> TSWSDRLQNAADMPANMDKHALKKYRREAYHRVFVNRSLAMEKIKCFGFNMDYTLAVYKSPEYESLGFELTVERLVSIGYPQELLSFAYDSTFPTRGLVFDTLYGNLLKVDAYGNLLVCAHGFNFIRGPETREQYPNKFIQRDDTERFYILNTLFNLPETYLLACLVDFFTNCPRYTSCETGFKDGDLFMSYRSMFQDVRDAVDWVHYKGSLKE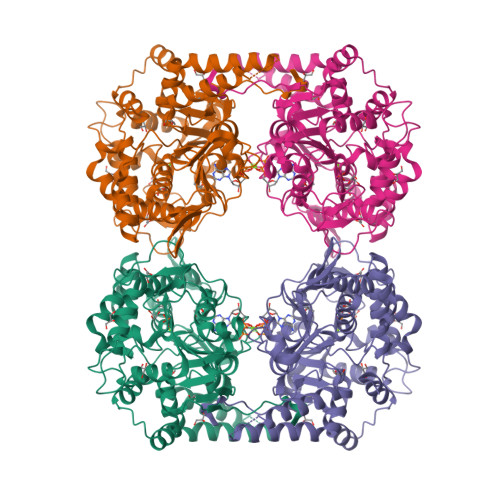KTVENLEKYVVKDGKLPLLLSRMKEVGKVFLATNSDYKYTDKIMTYLFDFPHGPKPGSSHRPWQSYFDLILVDARKPLFFGEGTVLRQVDTKTGKLKIGTYTGPLQHGIVYSGGSSDTICDLLGAKGKDILYIGDHIFGDILKSKKRQGWQTFLVIPELAQELHVWTDKSSLFEELQSLDIFLAELYKHLDSSSIQRRIKKVTHDMDMCYGMMGSLFRSGSRQTLFASQVMRYADLYAASFINLLYYPFSYLFRAAHVLMPHES>[6x]AFFTTVIIPAIVGGIATGTAVGTVSGLLGWGLKQAEEANKTPDKPDKVWRIQAGKGFNEFPNKEYDLYKSLLSSKIDGGWDWGNAATHYWIKGGQWNKLEVDMKDAVGTYKLSGLRNFTGGDLDVNMQKATLRLGQFNGNSFTSYKDSADRTTRVDFNAKNILIDNFLEINNRVGSGAGRKASSTVLTLQASEGITSSKNAEISLYDGATLNLASNSVKLNGNVWMGRLQYVGAYLAPSYSTINTSKVTGEVNFNHLTVGDHNAAQAGIIASNKTHIGTLDLWQSAGLNIIAPPEGGYKDKPNNTPSQSGAKNDKQESSQNNSNTQVINPPNSTQKTEVQPTQVIDGPFAGGKDTVVNIDRINTKADGTIKVGGFKASLTTNAAHLNIGKGGVNLSNQASGRTLLVENLTGNITVDGP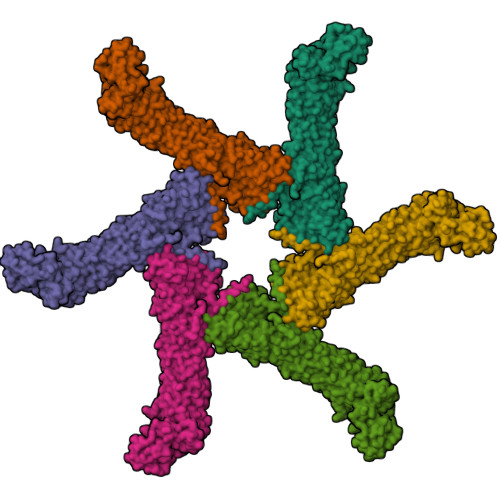LRVNNQVGGYALAGSSANFEFKAGVDTKNGTATFNNDISLGRFVNLKVDAHTANFKGIDTGNGGFNTLDFSGVTNKVNINKLITASTNVAVKNFNINELIVKTNGVSVGEYTHFSEDIGSQSRINTVRLETGTRSIFSGGVKFKSGEKLVIDEFYYSPWNYFDARNIKNVEITRKFASSTPENPWGTSKLMFNNLTLGQNAVMDYSQFSNLTIQGDFINNQGTINYLVRGGKVATLNVGNAAAMMFNNDIDSATGFYKPLIKINSAQDLIKNTEHVLLKAKIIGYGNVSTGTNGISNVNLEEQFKERLALYNNNNRMDTCVVRNTDDIKACGMAIGNQSMVNNPDNYKYLIGKAWKNIGISKTANGSKISVYYLGNSTPTENGGNTTNLPTNTTNNARFASYA>[3x]MGKSLSHLPLHSSKEDAYDGVTSENMRNGLVNSEVHNEDGRNGDVSQFPYVEFTGRDSVTCPTCQGTGRIPRGQENQLVALIPYSDQRLRPRRTKLYVMASVFVCLLLSG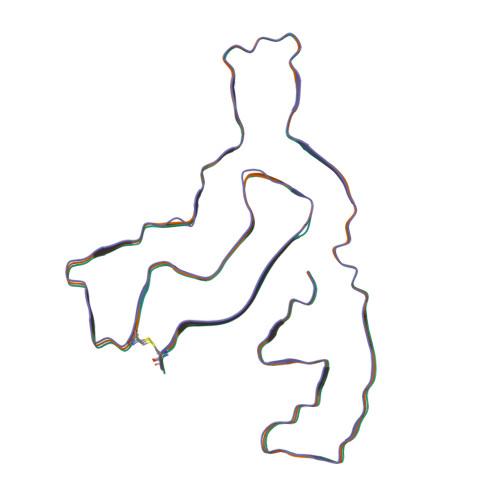LAVFFLFPRSIDVKYIGVKSAYVSYDVQKRTIYLNITNTLNITNNNYYSVEVENITAQVQFSKTVIGKARLNNITIIGPLDMKQIDYTVPTVIAEEMSYMYDFCTLISIKVHNIVLMMQVTVTTTYFGHSEQISQERYQYVDCGRNTTYQLGQSEYLNVLQPQQ N-benzyl-N-(2-{(4-cyanophenyl)[(1-methyl-1H-imidazol-5-yl)methyl]amino}ethyl)-1-methyl-1H-imidazole-4-sulfonamide 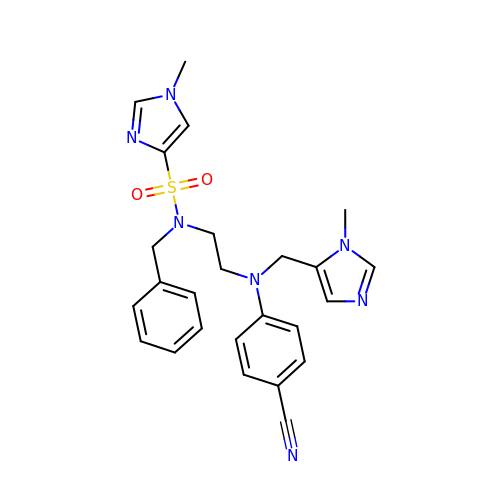| C25 H27 N7 O2 S | IDHGAQOVWWBGFK-UHFFFAOYSA-N>GVSEVRSDREKFTVYLDVKHFSPDELSVKVTDDYVEIQGKHGERQDDHGYISREFHRRYRLPSNVDQSAITCTLSAD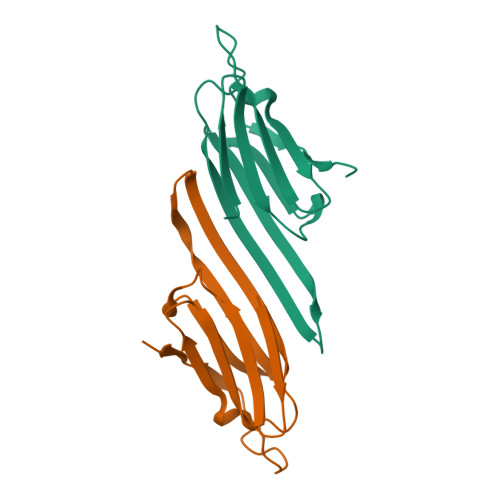GLLTLCGPKTSGIDAGRGDRTIPVTREDK[2x]>[2x]MSRLSEPSPYVEFDRRQWRALRMSTPLALTEEELVGLRGLGEQIDLLEVEEVYLPLARLIHLQVAARQRLFAATAEFLGEPQQNPDRPVPFIIGVAGSVAVGKSTTARVLQALLARWDHHPRVDLVTTDGFLYPNAE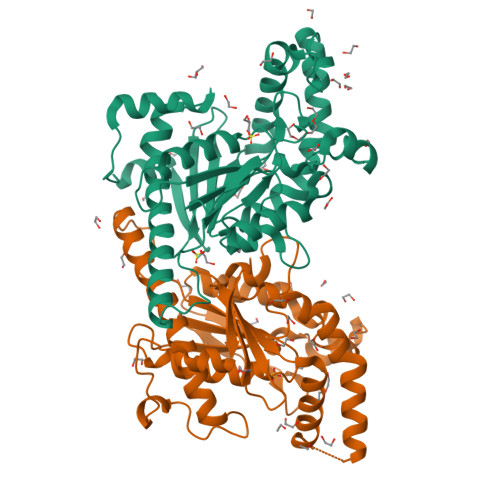LQRRNLMHRKGFPESYNRRALMRFVTSVKSGSDYACAPVYSHLHYDIIPGAEQVVRHPDILILEGLNVLQTGPTLMVSDLFDFSLYVDARIEDIEQWYVSRFLAMRTTAFADPESHAHHYAAFSDSQAVVAAREIWRTINRPNLVENILPTRPRATLVLRKDADHSINRLRLRKL>[6x]MRENNSGEKTRVLVVGGTGTMGRRIVRACLAEGHETYVLQQPETRVDIEKVQLLYSYKRLGARLIEASFSDHQSLVSAVKQVDIVVAAMSGVHFRSHSILVQLKLVEAIKEAGNIKRFLPSEFGMDPSRMGHAMPPGRETFDQKLEVRNAIEAAGIPHTYVVGACFAAYFAGNLSQMGTLIPPKKKVNIYGDGNVKVVYVDEDDIAEYTAKTLDDPRTINKTVYVRPTENVLTQMELVQIWEKLTGKELEKTNISANDFLADIEDKEIPHQAGLGHFYHIFYEGCLTDHEVGDDEEASKLYPDVKYTRMDEYLKIFL

Pinoresinol/lariciresinol reductase (PLR), an NADPH-dependent reductase, converts pinoresinol to lariciresinol and subsequently to secoisolariciresinol. Here, we present crystal structures of IiPLR1 from Isatis indigotica and pinoresinol reductases (PrRs) AtPrR1 and AtPrR2 from Arabidopsis thaliana, in the apo, substrate-bound and product-bound states. The crystal structures were captured in the apo, substrate-bound and/or product-bound forms. We found that, for all 16 structures we solved, each enzyme adopts a similar head-to-tail dimer conformation, strongly suggesting that each PLR/PrR functions as a homodimer, consistent with the literature that TpPLR1 exists as a dimeric entity in solution. Each structure contains a head-to-tail homodimer, and the catalytic pocket comprises structural elements from both monomers. β4 loop covers the top of the pocket, and residue 98 from the loop governs catalytic specificity.

Several regions (α5 loop, α9-helix, and α9 loop) are partially disordered both in the IiPLR1_apo and IiPLR1_NAP structures, for which the differences can be characterized by a RMSD of 0.287 Å, whereas the β4 loop is well defined in the apo structure. Intriguingly, the β4 loop is well defined in the AtPrR1_NAP structure but disordered in the AtPrR1/2_apo structures. These structural differences suggest that the loops are somewhat flexible, and act as a switch to control the binding of NADPH and release of NADP+. Residue Lys144, which corresponds to the previously reported Lys138 in TpPLR1 that serves as the general base for catalysis, forms direct hydrogen bonds with NADP+ in IiPLR1_apo and IiPLR1_NAP.>DYKDDDDKMDETELLRRSDGPVTRDRIRHDLAALGLVPGDTVMFHTRLSAIGYVSGGPQTVIDALLDVVGPTGTLLVTCGWNDAPPYDFTDWPPAWQEAVRAHHPAFDPRTSEAEHANGRLPEALRRRPGAVRSRHPDVSLAALGASAPALMDAHPWDDPHGPGSPLARLVALGGRVLLLGAPRDTMTLLHHAEALAQAPGKRFVTYEQPIEVAGERVWRTFRDIDSEHGAFDYSSAVPEGQDPFAVIVG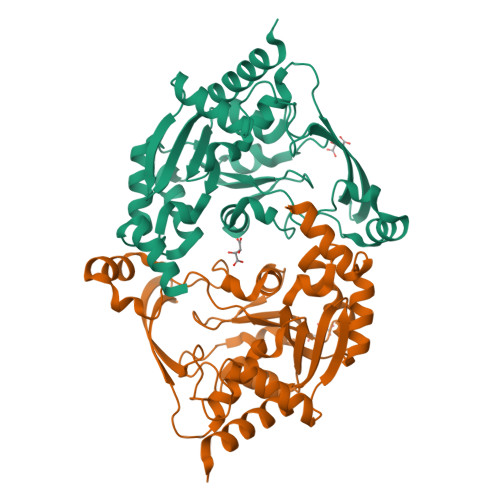SMLAAGIGREGFVGAARSRLFDAAPAVEFGVRWIEEHLNRDR[2x]> ESQPDPMPDDLHKSSEFTGTMGNMKYLYDDHYVSATKVKSVDKFLAHDLIYNINDKKLNNYDKVKTELLNEDLANKYKDEVVDVYGSNYY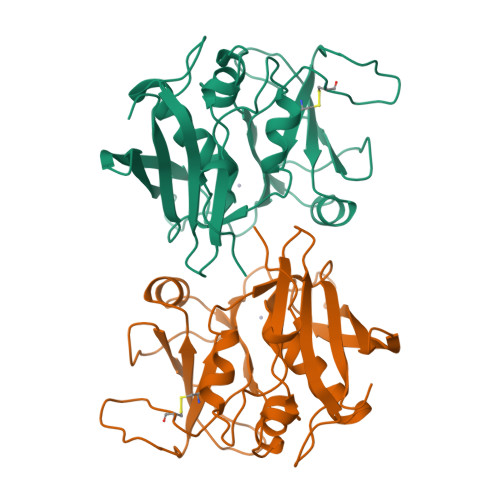VNCYFSSKDNVGKVTSGKTCMYGGITKHEGNHFDNGNLQNVLIRVYENKRNTISFEVQTDKKSVTAQELDIKARNFLINKKNLYEFNSSPYETGYIKFIESNGNTFWYDMMPAPGDKFDQSKYLMIYKDNKMVDSKSVKIEVHLTTKNG6-{[2-(dimethylamino)benzyl]amino}pyridine-3-carboxamide | C15 H18 N4 O | 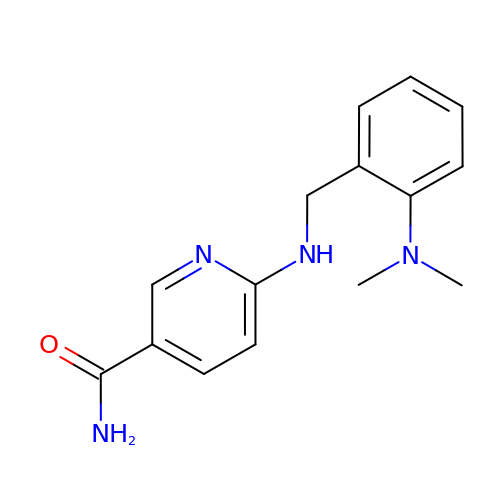OQZMUCDXSPWFIT-UHFFFAOYSA-N> MVKLAEFSRTATFAWSHDKIPLLVSGTVSGTVDANFSTDSSLELWSLLAADSEKPIASLQVDSKFNDLDWSHNNKIIAGALDNGSLELYSTNEANNAINSMARFSNHSSSVKTVKFNAKQDNVLASGGNNGEIFIWDMNKCTESPSNYTPLTPGQSMSSVDEVISLAWNQSLAHVFASAGSSNFASIWD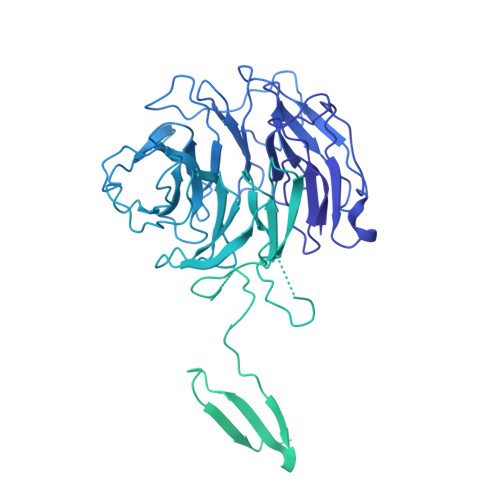LKAKKEVIHLSYTSPNSGIKQQLSVVEWHPKNSTRVATATGSDNDPSILIWDLRNANTPLQTLNQGHQKGILSLDWCHQDEHLLLSSGRDNTVLLWNPESAEQLSQFPARGNWCFKTKFAPEAPDLFACASFDNKIEVQTLQNLTNTLDEQETETKQQESETDFWNNVSREESKEKPSVFHLQAPTWYGEPSPAAHWAFGGKLVQITPDGKGVSITNPKISGLESNTTLSEALKTKDFKPLINQRLVKVIDDVNEEDWNLLEKLSMDGTEEFLKEALAFDNDESDAQDDANNEKEDDGEEFFQQIETNFQPEGDFSLSGNIEQTISKNLVSGNIKSAVKNSLENDLLMEAMVIALDSNNERLKESVKNAYFAKYGSKSSLSRILYSISKREVDDLVENLDVSQWKFISKAIQNLYPNDIAQRNEMLIKLGDRLKENGHRQDSLTLYLAAGSLDKVASIWLSEFPDLEDKLKKDNKTIYEAHSECLTEFIERFTVFSNFINGSSTINNEQLIAKFLEFINLTTSTGNFELATEFLNSLPSDNEEVKTEKARVLIASGKSLPAQNPATATTSKAKYTNAKTNKNVPVLPTPGMPSTTSIPSMQAPFYGMTPGASANALPPKPYVPATTTSAPVHTEGKYAPPSQPSMASPFVNKTNSSTRLNSFAPPPNPYATATVPATNVSTTSIPQNTFAPIQPGMPIMGDYNAQSSSIPSQPPINAVSGQTPHLNRKANDGWNDLPLKVKEKPSRAKAVSVAPPNILSTPTPLNGIPANAASTMPPPPLSRAPSSVSMVSPPPLHKNSRVPSLVATSESPRASISNPYAPPQSSQQFPIGTISTANQTSNTAQVASSNPYAPPPQQRVATPLSGGVPPAPLPKASNPYAPTATTQPNGSSYPPTGPYTNNHTMTSPPPVFNKPPTGPPPISMKKRSNKLASIEQNPSQGATYPPTLSSSASPLQPSQPPTLASQVNTSAENVSHEIPADQQPIVDFLKEELARVTPLTPKEYSKQLKDCDKRLKILFYHLEKQDLLTQPTIDCLHDLVALMKEKKYKEAMVIHANIATNHAQEGGNWLTGVKRLIGIAEATLN>[8x]SSSSAS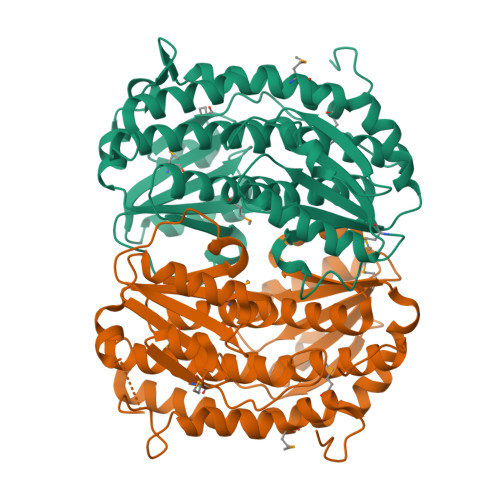KDGYKHYMLKEIYEQPEAVSNTILASLADGEISLDSFDKRAKELFEKTKHICIVACGTSYNAGMTAKYWIEKYAKVPCSVEIASEIRYRDNVVVDGSLFVSISQSGETADTLESLRKSKKQNYVGSMCICNVPNSSLVRESDIAFMTKAGVEIGVASTKAFTTQLVALAIFTLVIAKLKNSLTDQQIAKYTEELKNIRALVMGALKLDTEIDQISEYFSDKEHTIFLGRGLYYPIAIEGALKLKEISYIHAEAYPSGELKHGPLALVDKNMPIVAVVPNDELLDKTLSNLQEVHARGGKLILFVDKAVKERVNFDNSIVLELDAGHDFSAPVVFTIPLQLLSYHVAIIKGTDVDQPRNLAKSVTVE4-[8-methyl-3-[(4-methylphenyl)amino]imidazo[1,2-a]pyridin-2-yl]phenol | C21 H19 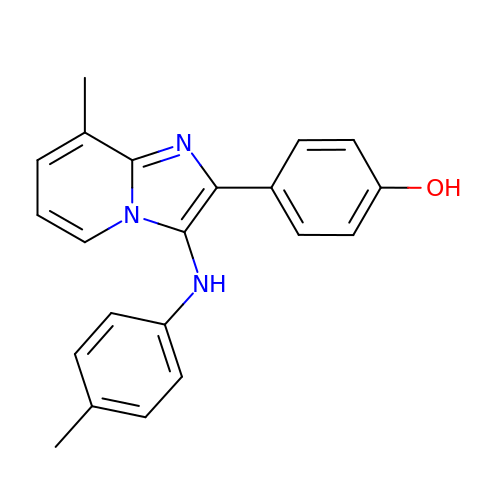N3 O | KPRSGDIGCGTRAS-UHFFFAOYSA-N>SNARRDKLKAQIAASGLDAMLISDLINVRYLSGFSGSNGALLVFADERDAVLATDGRYRTQAASQAPDLEVAIERAVGRYLAGRAGEAGVGKLGFESHVVTVDGLDALAGALEGKNTELVRASG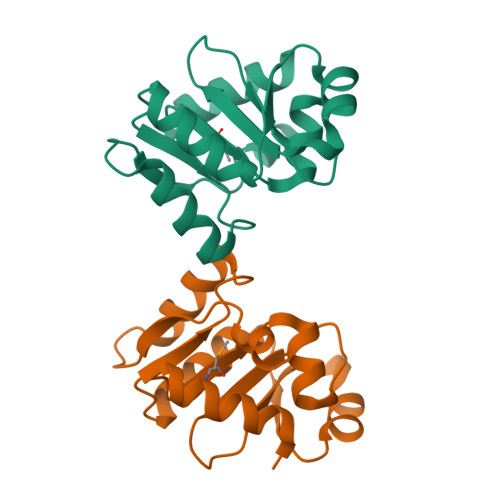TVESLREV[2x]>MHHHHHHSSGRENLYFQGDPRRRNILRSLRRNTKKPKPKPRPSITKATWESNYFGVPLTTVVTPEKPIPIFIERCIEYIEATGLSTEGIYRVSGNKSEMESLQRQFDQDHNLDLAEKDFTVNTVAGAMKSFFSELPDPLVPYNMQIDLVEAHKINDREQKLHALKEVLKKFPKENHEVFKYVISHLNKVSHNNKVNLMTSENLSICFWPTLMRPDFSTMDALTATRTYQTIIELFIQQCPFFFYNR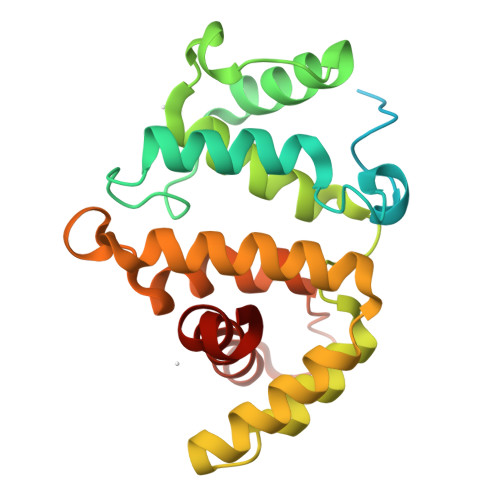[4x]Gene expression in the IncP-1 plasmids is stringently controlled by a network of four global repressors, KorA, KorB, TrbA and KorC interacting cooperatively. KorA is a 101-amino acid, homodimeric, protein with an N-terminal DNA-binding domain (DBD), containing a helix-turn-helix motif, and a C-terminal dimerization region, joined by a linker of four amino acids. In this study, we have determined the structures of the free KorA repressor and two complexes each bound to a 20-bp palindromic DNA duplex containing its consensus operator sequence. The structure of KorA consists of two domains, joined by a highly flexible, four amino acid linker, which retains its mobility even when bound to DNA.

KorA was crystallized in the presence of the operator OA. Structures from two of these were determined. Both show the DBDs of the protein symmetrically placed about the DNA axis. In contrast, the orientation of the CTD differs in the two crystal structures. In contrast to most proteins containing a helix-turn-helix motif, that bind to one face of the DNA; the two DBDs of KorA straddle the DNA, with helix 4 of the two subunits binding to opposite faces of the major groove. In each operator half site, five of the six consensus base pairs form direct hydrogen bonds to a protein side chain. In addition R48, at the beginning of helix 4, binds to Guanine 5 O6, but an alternative conformation of its sidechain is also seen in one half site, binding to phosphate 4. G49 is positioned so that its Cα atom is in van der Waal's contact with Thymine 7-O4. This restricts both the amino acid identity and the base, as other bases, including Cytosine, would cause a steric clash. The hydroxyl group of T47 forms a water-mediated contact with Adenine 13 in both chains. The remaining protein–DNA contacts are to the phosphate groups, including many from residues 18–23, outside the helix-turn-helix motif.

>MKKRLTESQFQEAIQGLEVGQQTIEIARGVLVDGKPQATFATSLGLTRGAVSQAVHRVWAAFEDKNLPEGYARVTAVLPEHQAYIVRKWEADAKKKQ[2x]>[2x]SFLLPKLTSKKEVDQAIKSTAEKVLVLRFGRDEDPVCLQLDDILSKTSSDLSKMAAIYLVDVDQTAVYTQYFDISYIPSTVFFFNGQHMKVDYGSPDHTKFVGSF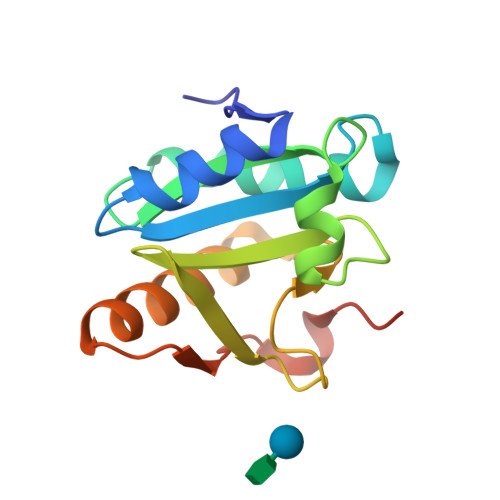KTKQDFIDLIEVIYRGAMRGKLIVQSPIDPKNIPKYDLLYQDI> GPDSASMAAERKTKLSKNLLRMKFMQRGLDSETKKQLEEEEKKIISEEHWYL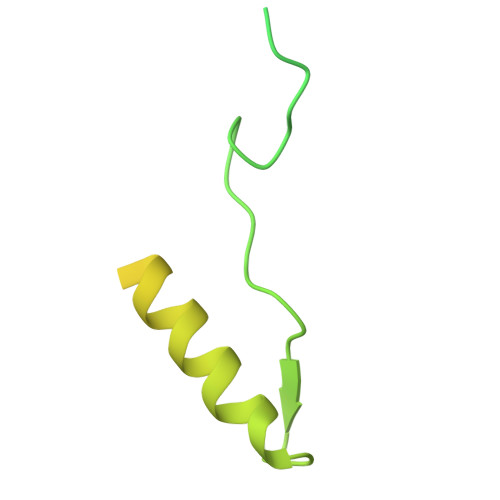DLPELKEKESFIIEEQSFLLCEDLLYGRMSFRGFNPEVEKLMLQMNAKHKAEEVEDETVELDVSDEEMARRYETLVGTIGKKFARKRDHANYEEDENGDITPIKAKKMFLKPQD Guanidinium | C H6 N3 | 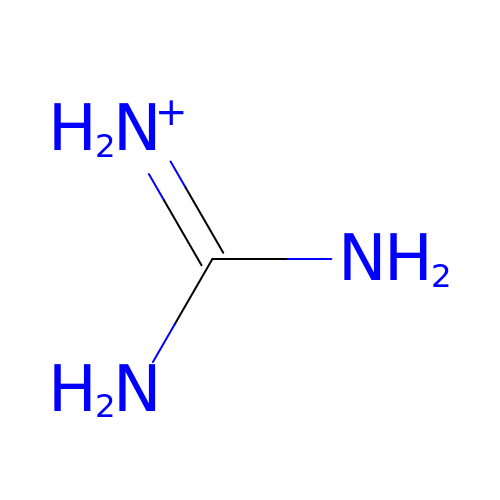ZRALSGWEFCBTJO-UHFFFAOYSA-O>MMSTTLFKDFTFEAAHRLPHVPEGHKAGRLHGHSFMVRLEITGEVDPHTGWIIDFAELKAAFKPTYERLDHH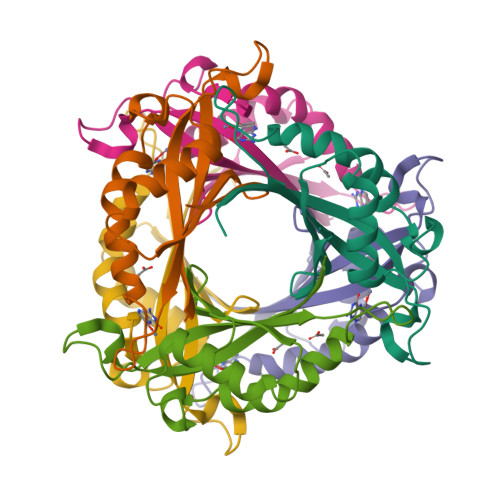YLNDIPGLENPTSEVLAKWIWDQVKPVVPLLSAVMVKETCTAGCIYRGE[6x]>[2x]MVIELTPSNFNREVIQSDSLWLVEFYAPWCGHCQRLTPEWKKAATALKDVVKVGAVDADKHHSLGGQYGVQGFPTIKIFGSNKNRPEDYQGGRTGE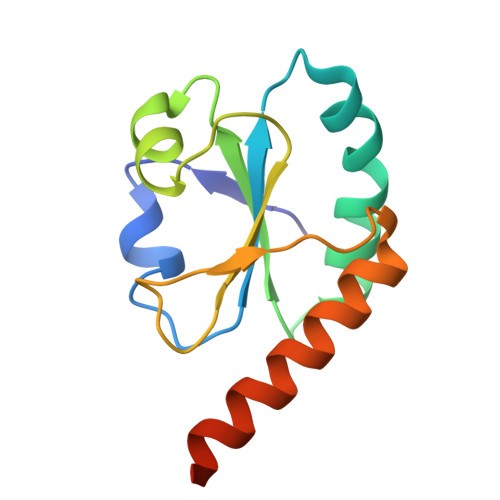AIVDAALSALRQLVKDRLGLEHHHHHH>[3x]MKTIKDRIAKWSAIGLLSAVAATAFYAPSASAHGEKSQAAFMRMRTIHWYDLSWSKEKVKINETVEIKGKFHVFEGWPETVDEPDVAFLNVGMPGPVFIRKESYIGGQLVPRSVRLEIGKTYDFRVVLKARRPGDWHVHTMMNVQGGGPIIGPGKWITVEGSMSEFRNPVTTLTGQTVDLENYNEGNTYFW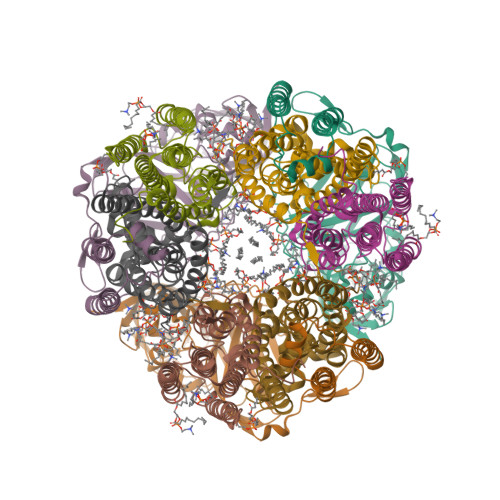HAFWFAIGVAWIGYWSRRPIFIPRLLMVDAGRADELVSATDRKVAMGFLAATILIVVMAMSSANSKYPITIPLQAGTMRGMKPLELPAPTVSVKVEDATYRVPGRAMRMKLTITNHGNSPIRLGEFYTASVRFLDSDVYKDTTGYPEDLLAEDGLSVSDNSPLAPGETRTVDVTASDAAWEVYRLSDIIYDPDSRFAGLLFFFDATGNRQVVQIDAPLIPSFM;>MSAAQSAVRSHAEAVQVSRTIDWMALFVVFFVIVGSYHIHAMLTMGDWDFWSDWKDRRLWVTVTPIVLVTFPAAVQSYLWERYRLPWGATVCVLGLLLGEWINRYFNFWGWTYFPINFVFPASLVPGAIILDTVLMLSGSYLFTAIVGAMGWGLIFYPGNWPIIAPLHVPVEYNGMLMSIADIQGYNYVRTGTPEYIRMVEKGTLRTFGKDVAPVSAFFSAFMSILIYFMWHFIGRWFSNERFLQST[3x];>MAATTIGGAAAAEAPLLDKKWLTFALAIYTVFYLWVRWYEGVYGWSAGLDSFAPEFETYWMNFLYTEIVLEIVTASILWGYLWKTRDRNLAALTPREELRRNFTHLVWLVAYAWAIYWGASYFTEQDGTWHQTIVRDTDFTPSHIIEFYLSYPIYIITGFAAFIYAKTRLPFFAKGISLPYLVLVVGPFMILPNVGLNEWGHTFWFMEELFVAPLHYGFVIFGWLALAVMGTLTQTFYSFAQGGLGQSLCEAVDEGLIAK[3x]>MYFFSVDPRNGASKSGDVCGSCCCESISARPGEVNGVMVSYAAWSAPLRGHGLTNKTTFEIDGVSVTPPKVSNAFGRTKVGVVFEGTLSDLFPNPEGEQVEYEISELNGPSNGVVELGANGAFTYTPGALFTGVDRFWFSINGNIGEYVISVDPTTSELPQPPFTTPVYVPAARRSVDPRTHVLKFVLGVSPAAIPGDVYRLTVRQVAIDCDGNEFVHISCYDISIGSCG[60x];>MNLDTLLPLQTIREHAKCDDNPRVTDDLLKLYREAAFEAAELYTGLSFTPEKTIVEPIRLKGRRGKIILSATPIAGRPVVFYGGGLGSPLELIPRPGSNVLFFPYGSPDRFQTWGDCHTCDVESQLMATYVTGRRCENSVPAGIIIGILKLIAWNINNPGDEVMSVRNTLNANAQGLIGGTNNGAVISGAQDEWFRYRRVLL[5x];>MVKLNCRPLCQAPTASRLVSPPCFICRGVAPSAPVTPG[25x];>[5x]MDCRNLCGAAAPSRLVQPGCFICRGVAVSIPPAAPGPATSVFDTPPSTFSLRPDGTIIAGTGIRGDHASVGTDGTIEMFIVPFIGDVTGSELTHPYAVELQDGEELAIAFGVTLKSGYGARITEYYDVSLFLENGGNSKELTLQPANTKSGYVWSDGHGYNITDSDGDLHTVQNVTRPVWFEMTEPGIVGVIMEARYKATGLVSSSISITVNVTYAD;>MANKESELNGLDDIHSDIEKLSAHVEKFSDGMDEKYKELTARFDGVKGDNDAIRKAVADATKEYAELSAKHQFFTEELAAMKARLDTPIMRSQAELDDHDRKTAIQLQRNMHEFRGGDPKEFVADESNLVDLKAYRSAVRKMLKVGIESKERVIASMTDVERKAFEASTIGPAFFTPQVLALEVDCNIECASLLDLYGQIEVSRSTFTYMKIADYGQLGEYTCDAKCDAEFGEPGNIRHLEGKTYDYRGVFCFNRKNLQEANYDFLSFMIGAAQRSHRINRNQALMIGKGVNEPKGWLTENCFPVFQTLPVDVNGTSTPAFLAQDWRRFVTSFPAEYGEARSVMHQNVFGYLAAMVDANGRFLFGDGDLTFTPDLVRERIRISNCLPDPTEGNTKGGTGQDAFAAGSFVAAQAAWKTAFYAVEKRPMFFEQYEGGS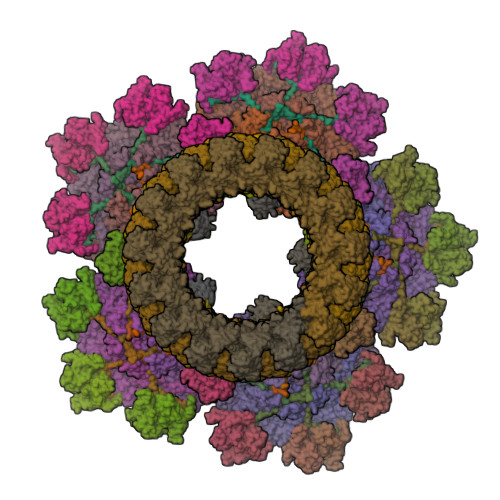SAWCVKYQFGAEDGGFVGCCEHGRILQIG[30x];>MNFNVGVDFPSFIAWDGEESFPVKVDGFNQFGFTFKTIAALTAATTFNIFYHEPSDADPCVPGPAIRVPEVPFCDTVLLSEDGLAAVTLPETVTPDSFCAGTVPCMNGQWISIAPATGSETNAANVQITVTMKGATR[40x]Here, we presented the X-ray structures of dimeric KillerOrange and monomeric mKillerOrange, the only known to date GFP-photosensitizers with Trp-based chromophore. To further expand the toolkit of available phototoxic proteins we have very recently come up with a blue-shifted KillerRed variant carrying tryptophan-based chromophore (substitutions: Gly3Cys, Tyr66Trp, Asp113Ser, Asn145Ser, Phe177Leu, Tyr221His, Glu236Gln) named KillerOrange. We also constructed monomeric mKillerOrange by introduction of the single Tyr66Trp substitution in SuperNova, a monomeric variant of KillerRed. The principal structural fold of the monomer in KillerOrange/mKillerOrange, shared with all members of the GFP family, is an 11-stranded β-barrel having loops from both sides and the chromophore (matured from Gln65-Trp66-Gly67 sequence) embedded in the middle of the internal α-helix wound around the β-barrel axis.

The crystal asymmetric unit of KillerOrange contains two dimers and one monomer forming a dimer with the symmetry related subunit, while the crystal asymmetric unit of mKillerOrange contains one monomer. Similar to parental SuperNova, destabilization of central hydrophobic patch in the dimeric KillerOrange by Leu160Thr and Phe162Thr replacements ensures a monomeric state of mKillerOrange. In the channel of mKillerOrange, we found a glycerol molecule, presumably coming from the cryoprotecting solution and replacing three out of seven water molecules present in KillerOrange. The side chain of Trp66 of the chromophore in KillerOrange and mKillerOrange adopts an unusual trans-cis conformation, not seen for other Trp-based chromophores before. It is described by the χ1/χ2 torsion angles of 175°/16° and -178°/26°, respectively (rotation around Cα-Cβ and Cβ-Cγ bonds defined by dihedral angles N-Cα-Cβ- Cγ and Cα-Cβ-Cγ-Cδ). A higher resolution structure of mKillerOrange also shows the traces (~10–15%) of alternative cis-cis conformation with χ1/χ2 of -5°/-8°. In both structures, the indole ring of Trp66 in a dominant trans-cis conformation is stabilized by hydrogen bond between the indole nitrogen and the side chain of Gln159 and shows a noticeable deviation from the chromophore planarity (χ2 ~16–26°). Conversely, in the minor cis-cis conformation the indole ring is nearly coplanar with the chromophore imidazolinone ring and is stabilized by a hydrogen bond with Thr201. In both proteins, the nearest environment of the QWG chromophore (within 3.9 Å) is nearly identical and consists of 19 residues with the only difference at position 177 occupied by Leu and Phe in KillerOrange and mKillerOrange, respectively. Similar to their red progenitors, KillerOrange and mKillerOrange, show the presence of a water-filled channel extending along the β-barrel axis.

> MRGSHHHHHHGSRGSEVGPALFQSDMTFKIFIDGEVNGQKFTIVADGSSKFPHGDFNVHAVCETGKLPMSWKPICHLIQWGEPFFARYPDGISHFAQECFPEGLSIDRTVRFENDGTMTSHHTYELDDTCVVSRITVNCDGFQPDGPIMRDQLVDILPSETHMFPHGPNAVRQTATIGFTTADGGKMMGHFDSKMTFNGSRAIEIPGPHFVTIITKQTRDTSDKRDHVCQREVAYAHSVPRI(2R)-1-{[(2,6-dichlorophenyl)methyl]amino}propan-2-ol | C10 H13 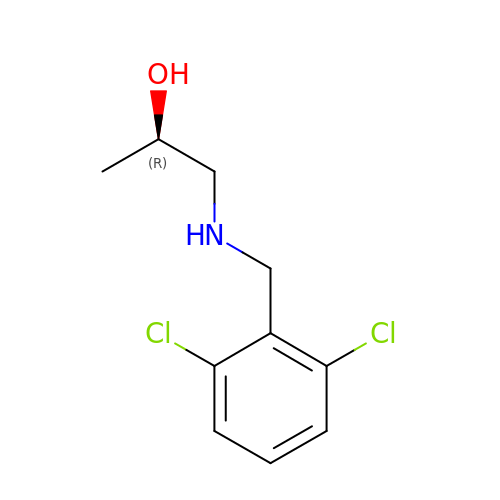Cl2 N O | BNJMFYUVZZATLR-SSDOTTSWSA-N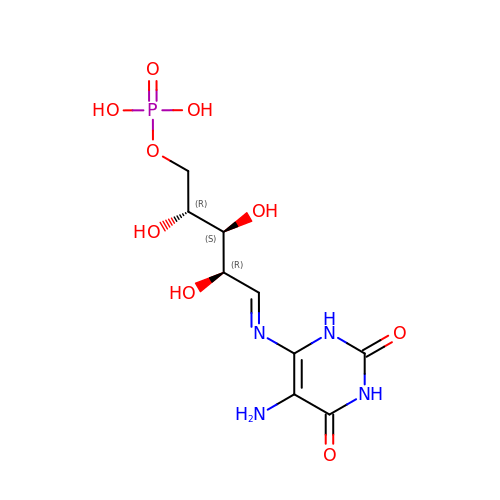[(2R,3S,4R,5E)-5-[(5-amino-2,6-dioxo-3H-pyrimidin-4-yl)imino]-2,3,4-trihydroxy-pentyl] dihydrogen phosphate | C9 H15 N4 O9 P | XKTZRTIKRCUGRX-QNGFKNCYSA-N>[2x]GPLGSDYIIKEKTVLLQKKDSEGFGFVLRGAKAQTPIEEFTPTPAFPALQYLESVDEGGVAWRAGLRMGDFLIEVNGQNVVKVGHRQVVNMIRQGGNTLMVKVVMVTRHPDM;>TRL[2x]

As a model β-strand mediated PPI, we use the GKAP/SHANK-PDZ50 which, plays a role in the organization of synaptic protein complexes and has been linked to several neuronal disorders. There are >250 PDZ domains with several therapeutically relevant proteins known to exhibit their function through a PDZ mediated interaction. Class I PDZ domains bind to consensus sequences with a Thr/Ser in the -2 position from the C-terminus, with the C-terminus hydrophobic residue and free carboxylate being the main determinants of affinity. Here, we used dynamic ligation screening to identify peptide-fragment hybrids linked through an acylhydrazone bond, that are able to functionally mimic a β-strand and inhibit its PPI using GKAP/SHANK1 PDZ as a model interaction.

Interestingly, the most potent hybrids formed from 3 and 4 contained the same carboxylic acid functionalized aromatic aldehyde fragments (A047 and A048), indicating that these types of fragments might play an important role in binding. In all hybrids, the hydrazone bond existed in an E configuration with the aromatic ring of the fragment co-planar with the hydrazone. Although this leads to slight uncertainty about the exact location of the fragments, we hypothesize that the key carboxylic acid moiety moves dynamically across a positively charged patch formed by R679, R736 and R743 on the protein surface, making transient charge-reinforced hydrogen-bonding and cation–π interactions which is also consistent with a more favourable entropy of interaction. To provide support for the hypothesis that the hybrids target the cationic patch on the surface of SHANK1, we performed molecular dynamics simulations on the SHANK1-compound 3-A048 complex using the crystal structure as a starting point. Over the course of three repeats of 200 ns, the aromatic carboxylate of the fragment indeed moves across the surface of the SHANK1 protein, making transient contacts with R679, R736 and R743, as well as intramolecular interaction onto the arginine in the peptide ligand to a lesser extent (see: ESI, Movie S1†). The distance between the carboxylate and these residues plotted against time over the course of the simulations (Fig. S21†) further indicates that the aromatic carboxylate is able to make transient non-covalent contacts in turn with each of the positively charged side-chains of the three arginine residues with a preference for R736.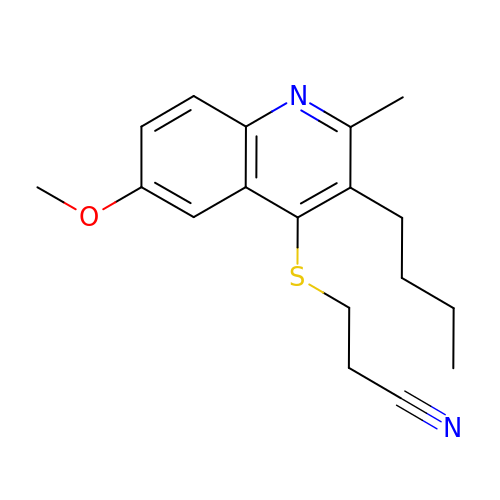3-(3-BUTYL-6-METHOXY-2-METHYL-QUINOLIN-4-YL)SULFANYLPROPANENITRILE | C18 H22 N2 O S | UJFIVLIFWNFOIZ-UHFFFAOYSA-N(4-{2-ACETYLAMINO-2-[1-(3-CARBAMOYL-4-CYCLOHEXYLMETHOXY-PHENYL)-ETHYLCARBAMOYL}-ETHYL}-2-PHOSPHONO-PHENOXY)-ACETIC ACID | C29 H38 N3 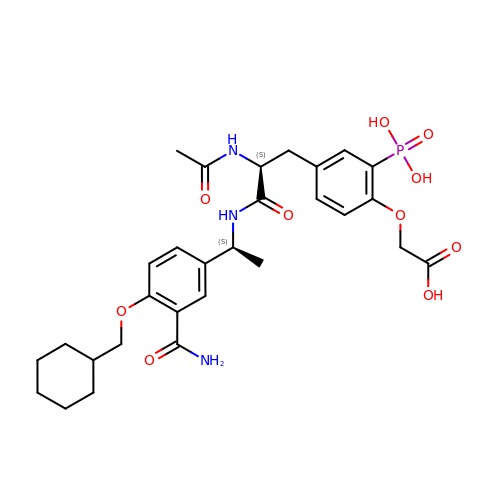O10 P | FXUGQWABROMTDA-SBUREZEXSA-N>SIPETQKGVIFYESHGKLEYKDIPVP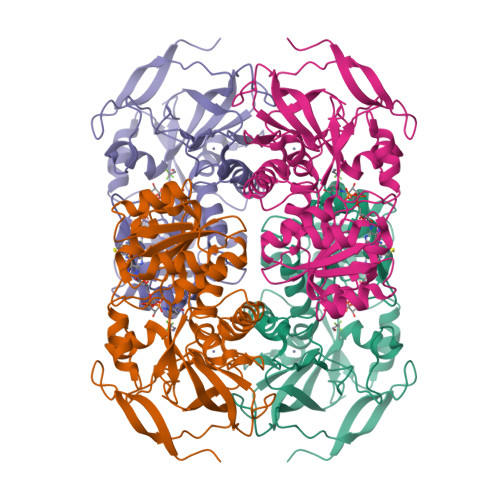KPKANELLINVKYSGVCHTDLHAWHGDWPLPVKLPLVGGHEGAGVVVGMGENVKGWKIGDYAGIKWLNGSCMACEYCELGNESNCPHADLSGYTHDGSFQQYATADAVQAAHIPQGTDLAQVAPILCAGITVYKALKSANLMAGHWVAISGAAGGLGSLAVQYAKAMGYRVLGIDGGEGKEELFRSIGGEVFIDFTKEKDIVGAVLKATDGGAHGVINVSVSEAAIEASTRYVRANGTTVLVGMPAGAKCCSDVFNQVVKSISIVGSYVGNRADTREALDFFARGLVKSPIKVVGLSTLPEIYEKMEKGQIVGRYVVDTSK[4x]> GPLGSLFRSLVGTSRAIQ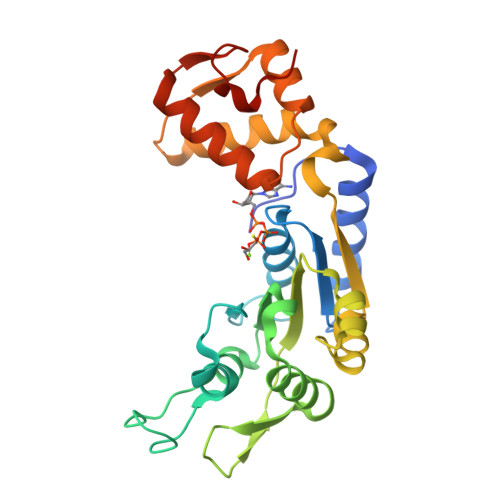QVRQMMQQVADTDASVLILGESGTGKEVVARNLHYHSKRREGPFVPVNCGAIPAELLESELFGHEKGAFTGAITSRAGRFELANGGTLFLDEIGDMPLPMQVKLLRVLQERTFERVGSNKTQNVDVRIIAATHKNLEKMIEDGTFREDLYYRLNVFPIEMAPLRERVEDIALLLNELISRMEHEKRGSIRFNSAAIMSLCRHDWPGNVRELANLVERLAIMHPYGVIGVGELPKKFRHVDDEDEQ>[2x]GSHMSTNKITFLLNWEAAPYHIPVYLANIKGYFKDENLDIAILEPSNPSDVTELVGSGKVDMGLKAMVGTLAAKARGFPVTSIGSLLDEPFTGICYLEGSGITSDFQSLKGKRIGYVGEFGKIQVDELTKHYGMTPDDYVAVRCGMNVAKYILEGTIDCGIGIECIQQVELEEALKEQGKDSNDAKMLRIDKLAELGCCCF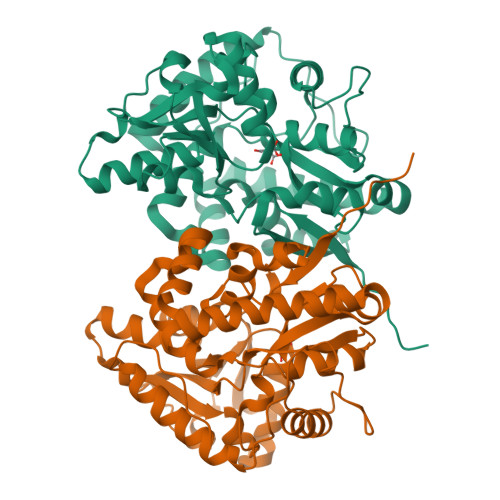CTILYIANDKFIAENPQAVKKFLKAIKRATDYMLAHPREAWAEYGNFKPTMQTDLNTKKFQRCYAYFSESLYNVHRDWRKVNNYGKRLDILPENYVPNYTNEYLSWPEPKEVDDPEKAQDLMLKHQEECKTCGGYKRLVLA>MFDTSPRLDCAGRILTLDRPRVMGIVNVTPDSFSDGGTHTTVEAAVAHGLRLAEEGADLLDIGGESTRPGATAVPVEEELRRVIPVIERLVAQTALPLSVDTFKPEVMRAAVAAGAGMINDVQALRQPGALDAVADLRVPVVLMHMPGDAYAAGSAPHYDDVVAEVHRFLVERIFAAEMAGIDKRRLLIDPGFGFGKSTAD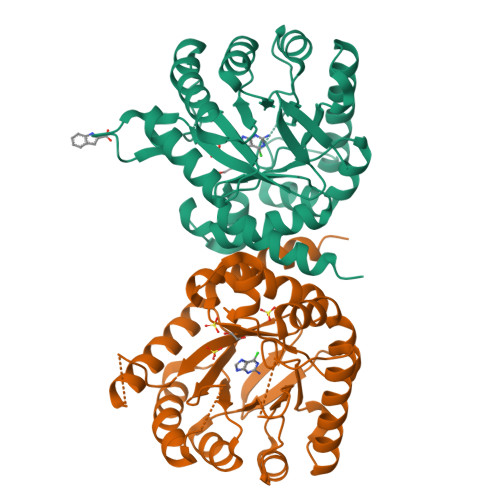NVQLLAHLPRLCELGVPVLAGLSRKRSIGELTGRELPEQRVAGSVAAHLLAAQRGALLLRVHDVAATVDALTVWQAVQAVPSPRVATGTAMPIRWPDED[4x]> APKDNHHHHHHANKEATRNAAALFSVDYKAFLNEVSNLNKRMGDLRDINGEAGAWARIMSGTGSASGGFSDNYTHVQVGVDKKHELDGLDLFTGFTVTHTDSSASADVFSGKTKSVGAGLYASAMFDSGAYIDLIGKYVHHDNEYTATFAGLGTRDYSTHSWYAGAEAGYRYHVTEDAWIEPQAELVYGSVSGKQFAWKDQGMHLSMKDKDYNPLIGRTGVDVGKSFSGKDWKVTARAGLGYQFDLLANGETVLRDASGEKRIKGEKDSRMLMSVGLNAEIRDNVRFGLEFEKSAFGKYNVD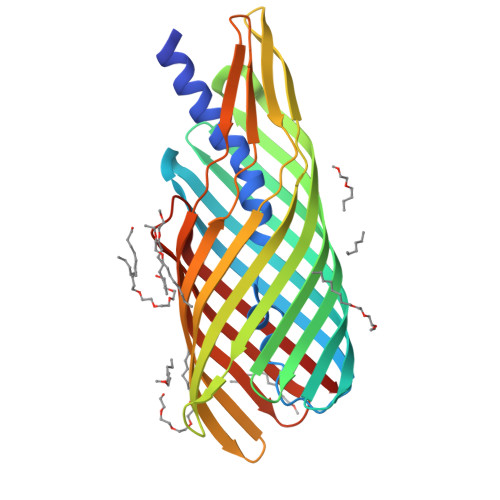NAVNANFRYSF>[3x]TLSEKIHHPITEQGGESDLSSFAPDAASITSSIKYHAEFTPVFSP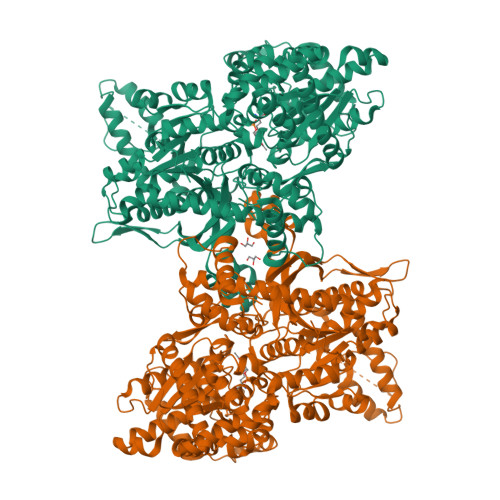ERFELPKAFFATAQSVRDSLLINWNATYDIYEKLNMKQAYYLSMEFLQGRALLNAIGNLELTGAFAEALKNLGHNLENVASQEPDAALGNGGLGRLASCFLDSLATLNYPAWGYGLRYKYGLFKQRITKDGQEEVAEDWLEIGSPWEVVRNDVSYPIKFYGKVSTGSDGKRYWIGGEDIKAVAYDVPIPGYKTRTTISLRLWSTQVPSADFDLSAFNAGEHTKACEAQANAEKICYILYPGDESEEGKILRLKQQYTLCSASLQDIISRFERRSGDRIKWEEFPEKVAVQMNDTHPTLCIPELMRILIDLKGLNWNEAWNITQRTVAYTNHTVLPEALEKWSYELMQKLLPRHVEIIEAIDEELVHEIVLKYGSMDLNKLEEKLTTMRILENFDLPSSVAELFIKPEISVDDDTETVEVHDKVEASDKVVTNDEDDTGKKTSVKIEAAAEKDIDKKTPVSPEPAVIPPKKVRMANLCVVGGHAVNGVAEIHSEIVKEEVFNDFYELWPEKFQNKTNGVTPRRWIRFCNPPLSAIITKWTGTEDWVLKTEKLAELQKFADNEDLQNEWREAKRSNKIKVVSFLKEKTGYSVVPDAMFDIQVKRIHEYKRQLLNIFGIVYRYKKMKEMTAAERKTNFVPRVCIFGGKAFATYVQAKRIVKFITDVGATINHDPEIGDLLKVVFVPDYNVSVAELLIPASDLSEHISTAGMEASGTSNMKFAMNGCIQIGTLDGANVEIREEVGEENFFLFGAQAHEIAGLRKERADGKFVPDERFEEVKEFVRSGAFGSYNYDDLIGSLEGNEGFGRADYFLVGKDFPSYIECQEKVDEAYRDQKRWTTMSILNTAGSYKFSSDRTIHEYAKDIWNIEAVEIA>IVGGYTCAANSIPYQVSLNSGSHFCGGSLINSQWVVSAAHCYKSRIQVRLGEHNIDVLEGNEQFINAAKIITHPNFNGNTLDNDIMLIKLSSPATLNSRVATVSLPRSCAAAGTECLISGWGNTKSSGSSYPSLLQCLKAPVLSDSSCKSSYPGQITGNMICVGFLEGGKDSCQGDSGGPVVCNGQLQGIVSWGYGCAQKNKPGVYTK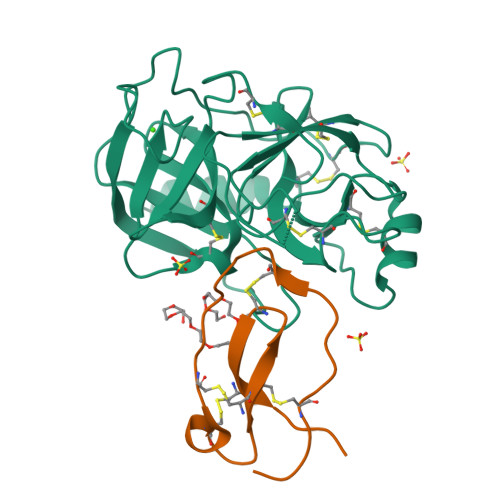VCNYVNWIQQTIAAN[3x];>KPGKCPVTYGQCLMLNPPNFCEMDGQCKRDLKCCMGMCGKSCVSPVK[2x]>[2x]STAGKVIKCKAAVLWEEKKPFSIEEVEVAPPKAHEVRIKMVATGICRSDDHVVSGTLVTPLPVIAGHEAAGIVESIGEGVTTVRPGDKVIPLFTPQCGKCRVCKHPEGNFCLKNDLSMPRGTMQDGTSRFTCRGKPIHHFLGTST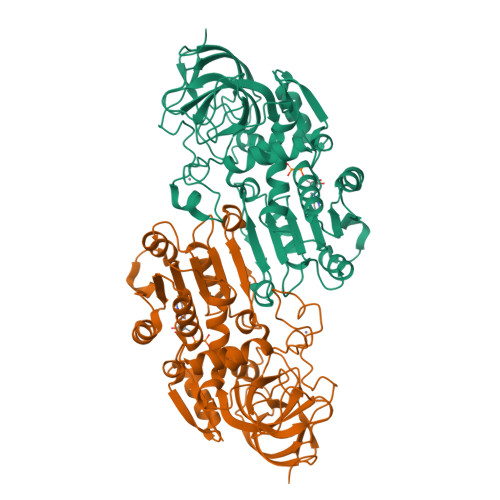FSQYTVVDEISVAKIDAASPLEKVCLIGCGFSTGYGSAVKVAKVTQGSTCAVFGLGGVGLSVIMGCKAAGAARIIGVDINKDKFAKAKEVGATECVNPQDYKKPIQEVLTEMSNGGVDFSFEVIGRLDTMVTALSCCQEAYGVSVISGVPPDSQNLSMNPMLLLSGRTWKGAIFGGFKSKDSVPKLVADFMAKKFALDPLITHVLPFEKINEGFDLLRSGESIRTILTF>MSTQDLSGKIALVTGASRGIGAAIADTLAAAGAKVIGTATSESGAAAISERLAQWGGEGRVLNSAEPETVENLIADIEKTFGKLDILVNNAGITRDNLLMRMKEEEWDDIMQVNLKSVFRASKAVLRGMMKQRAGRIINITSVVGVMGNAGQTNYAAAKAGLIGFSKSMAREVGSRGITVNCVAPGFIDTDMTRALPEETRQTFTAQTALGRFGDAQDIADAV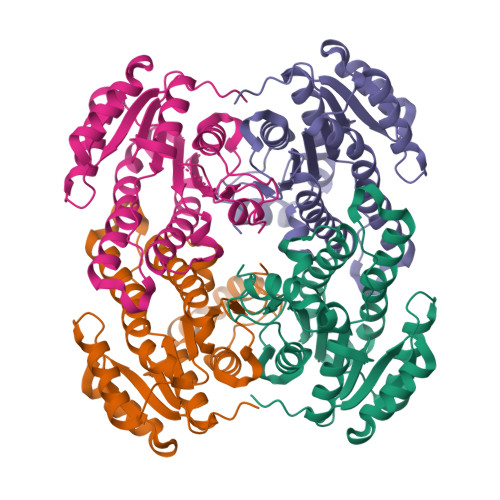LFLASDQAKYITGQTLHVNGGMLMP[4x]>[2x]MEQRFPELNV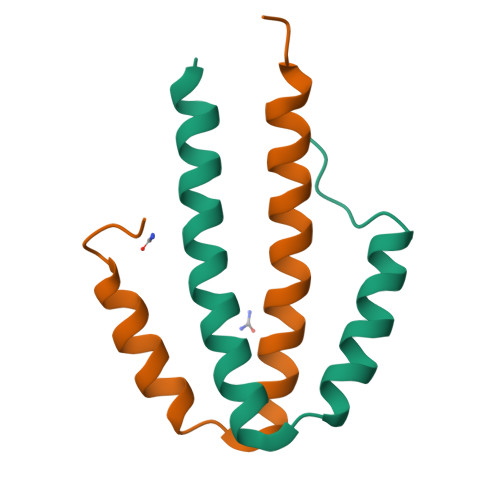DLSFEQEFQMRVMEEQVSAMSLQEARELLLQASRLLMMKDNVIRSLVKRAARS>MKLYYSPGACSLSPHIALREAGLNFELVQVDLASKKTASGQDYLEVNPAGYVPCLQLDDGRTLTEGPAIVQYVADQVPGKQLAPANGSFERYHLQQWLNFISSELHKSFSPLFNPASSDEWKNAVRQSLNTRLGQVARQLEHAPYLLGDQLSVADIYLFVVLGWSAYVNIDLSPWPSLQAFQGRV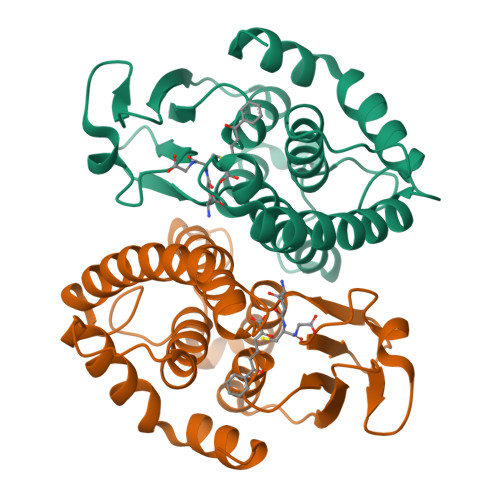GGREAVQSALRAEGLIKE[4x]> GSHMKPHPWFFGKIPRAKAEEMLSKQRHDGAFLIRESESAPGDFSLSVKFGNDVQHFKVLRDGAGKYFLWVVKFNSLNELVDYHRSTSVSRNQQIFLRDIE;> QNGYVNPT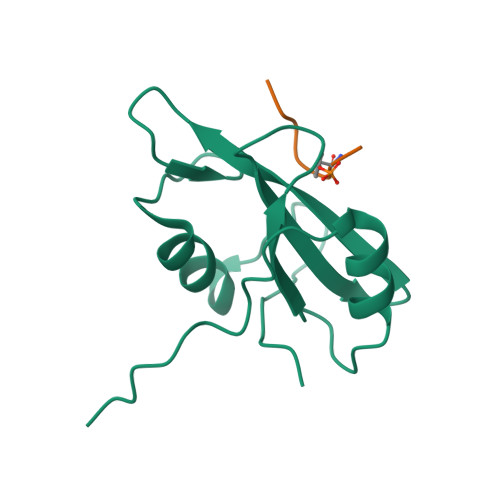Y> MKRIPRKTKGKSSGKGNDSTERADDGSSQLR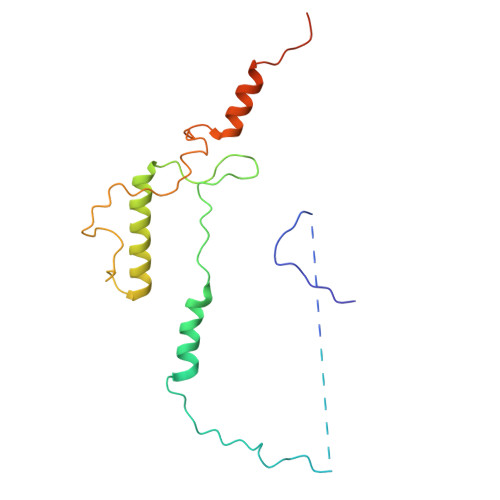DKQNNKAGPATTEPGTSNREQYKARPGIASVQRATESAEMPMKNNDEGTPDKKGNTKGDLVNEHSEAKDEADEATKKQAKDTDKSKAQVTYSDTGINNANELSRSGNVDNEGGSNQKPMSTRIAEATSAIVSKHPARVGLPPTASSGHG6-CARBOXYLYSINE | C7 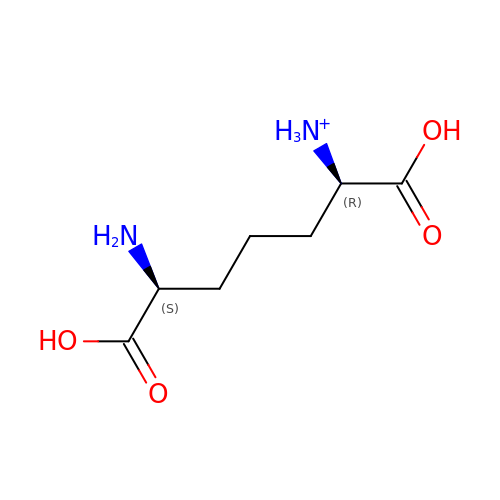H15 N2 O4 | GMKMEZVLHJARHF-SYDPRGILSA-O> SW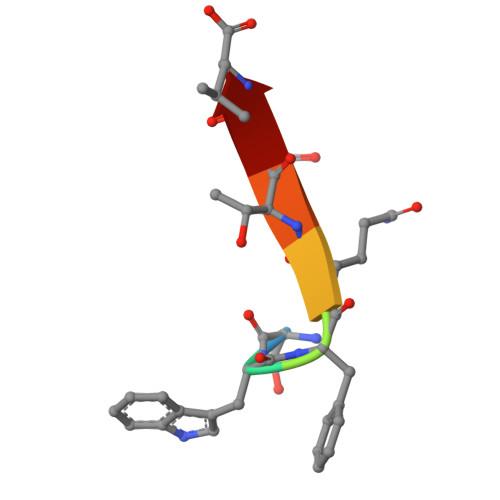FQTDL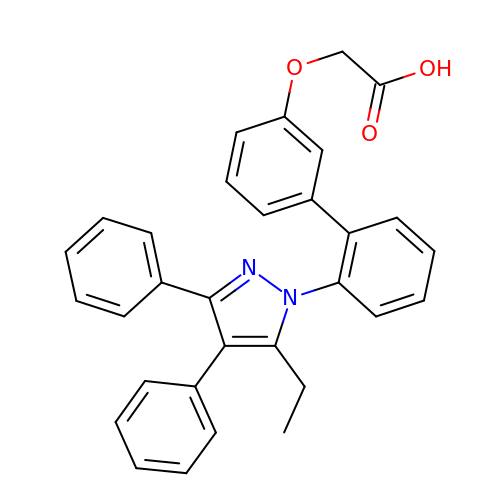((2'-(5-ETHYL-3,4-DIPHENYL-1H-PYRAZOL-1-YL)-3-BIPHENYLYL)OXY)ACETIC ACID | C31 H26 N2 O3 | SJRVJRYZAQYCEE-UHFFFAOYSA-N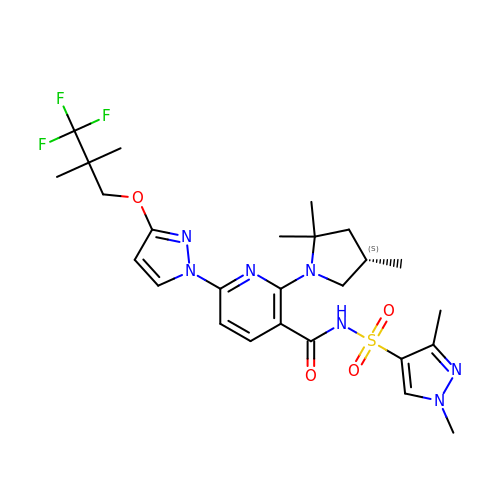(6P)-N-(1,3-dimethyl-1H-pyrazole-4-sulfonyl)-6-[3-(3,3,3-trifluoro-2,2-dimethylpropoxy)-1H-pyrazol-1-yl]-2-[(4S)-2,2,4-trimethylpyrrolidin-1-yl]pyridine-3-carboxamide | C26 H34 F3 N7 O4 S | MVRHVFSOIWFBTE-INIZCTEOSA-N> MVKQIESKTAFQEALDAAGDKLVVVDFSATWCGPCKMIKPFFHSLSEKYS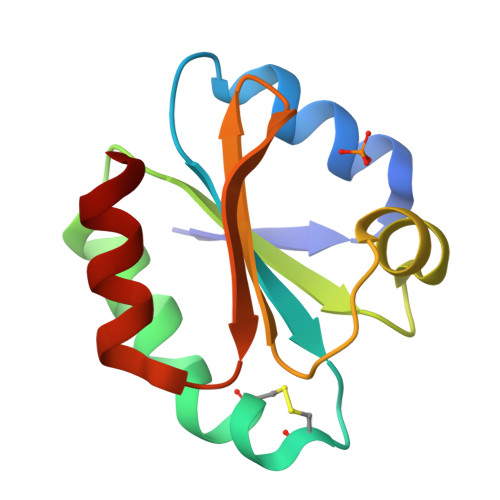NVIFLEVDVDDCQDVASECEVKSMPTFQFFKKGQKVGEFSGANKEKLEATINELV> MIIYRDLISHDEMFSDIYKIREIADGLCLEVEGKMVSGG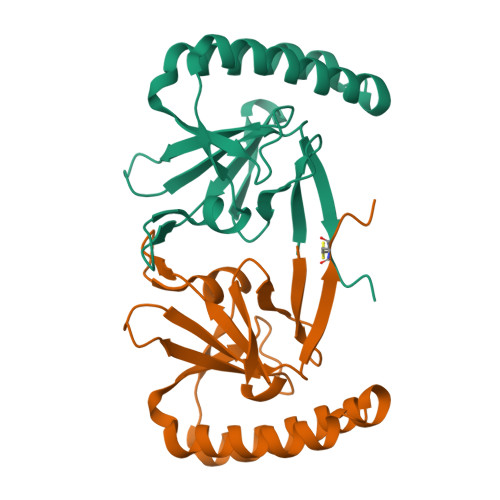ITGVDIVMNHHLQETSFTKEAYKKYIKDYMKSIKGKLEEQRPERVKPFMTGAAEQIKHILANFKNYQFFIGENMNPDGMVALLDYREDGVTPYMIFFKDGLEMEKCLEHHHHHH> IAGGEAITTGGSRCSLGFNVSVNGVAHALTAGHCTNISASWSIGTRTGTSFPNND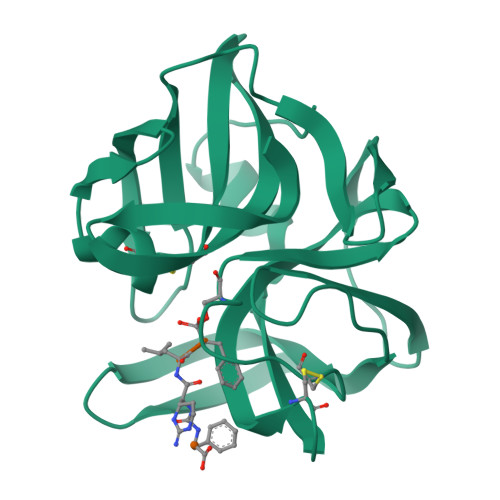YGIIRHSNPAAADGRVYLYNGSYQDITTAGNAFVGQAVQRSGSTTGLRSGSVTGLNATVNYGSSGIVYGMIQTNVCAQPGDSGGSLFAGSTALGLTSGGSGNCRTGGTTFYQPVTEALSAYGATVL> RIALYIGNLTWWTTDEDLTEAVHSLGVNDILEIKFFENRANGQ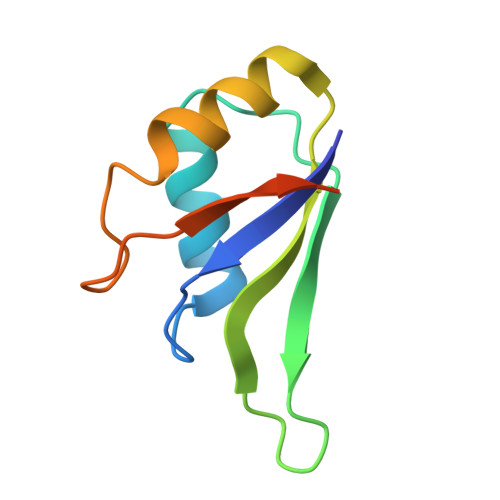SKGFALVGVGSEASSKKLMDLLPKRELHGQNPVVTPSNKLEHHHHHH>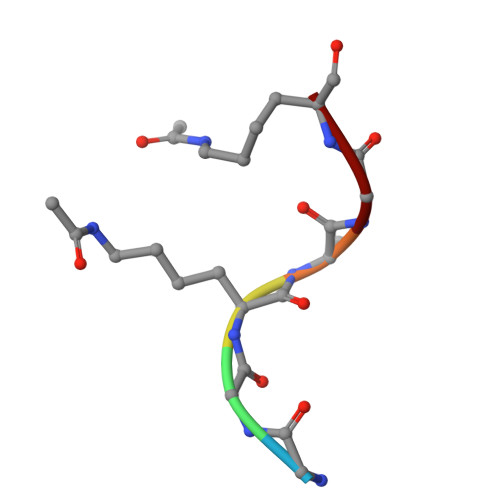 GGKAGK> STAFTGVRDVPAQQIVNEMKVGWNLGNT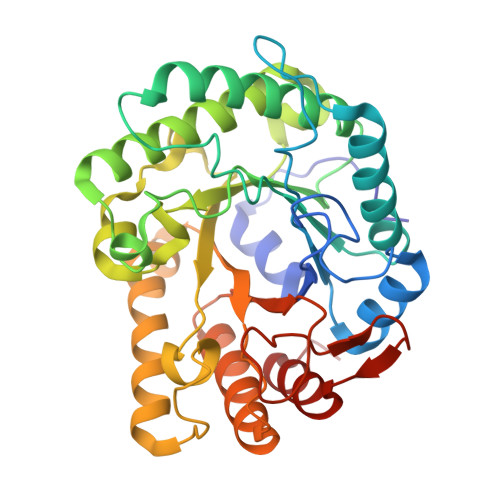MDAIGGETNWGNPMTTHAMINKIKEAGFNTLRLPVTWDGHMGAAPEYTIDQTWMKRVEEIANYAFDNDMYVIINLHHENEWLKPFYANEAQVKAQLTKVWTQIANNFKKYGDHLIFETMNEPRPVGASLQWTGGSYENREVVNRYNLTAVNAIRATGGNNATRYIMVPTLAASAMSTTINDLVIPNNDSKVIVSLHMYSPYFFAMDINGTSSWGSDYDKSSLDSEFDAVYNKFVKNGRAVVIGEMGSINKNNTAARVTHAEYYAKSAKARGLTPIWWDNGYSVAGKAETFGIFNRSNLTWDAPEVMKAFIKGIGGSS> MAAFRDIEEVSQGLLSLLGANRAEAQQRRLLGRHEQVVERLLETQDGAEKQLREILTMEKEVAQSLLNAKEQVHQGGVELQQLEAGLQEAGEEDTRLKASLLQLTRELEELKEIEADLERQEKEVDEDTTVTIPSAVYVAQLYHQVSKIEWDYECEPGMVKGI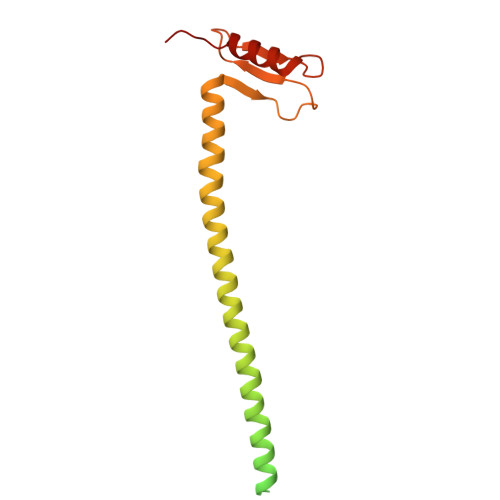HHGPSVAQPIHLDSTQLSRKFISDYLWSLVDTEW1,1'-ethane-1,2-diyldipyrrolidine-2,5-dione | C10 H12 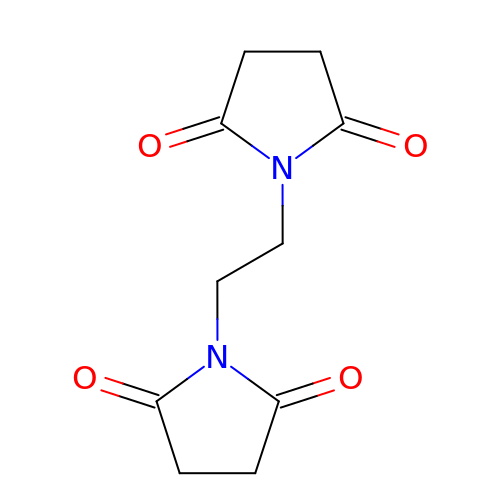N2 O4 | ZFMTZVFTWHQGNQ-UHFFFAOYSA-N Dye-decolorizing peroxidases (DyPs) are heme proteins with distinct structural properties and substrate specificities compared to classical peroxidases. Here, we demonstrate that DyP from the extremely radiation-resistant bacterium Deinococcus radiodurans is, like some other homologues, inactive at physiological pH. Structurally, DyP-type peroxidases also differ from the classical peroxidases. In contrast with the α-helix rich structures of the latter, DyPs are organized in two domains with a ferredoxin-like fold of four anti-parallel β-sheets surrounded by α-helices. A sequence analysis of DrDyP compared to four characterized and structurally determined members of the class V peroxidase family of DyPs, demonstrates that the proximal His heme ligand, and the four residues that are proposed to form the hydrogen peroxide binding pocket within this family of DyPs are conserved in DrDyP (H324, D189, R348, L373 and F375).

However, the so-called DyP fingerprint motif GXXDG has a substitution in the fifth position, containing a Methionine (M190) instead of a Glycine, as observed for the other DyPs. The proximity of this residue to the catalytic residue Asp189 made us suspect that it might affect the activity of the protein; we, thus, re-engineered a typical DyP distal site by generating the DrDyPM190G mutant for spectroscopic analysis. UV-vis and RR spectroscopies reveal that the resulting DrDyPM190G is also in a 6cLS spin state at pH 7.5, and thus the Methionine does not affect the activity of the protein. The E°′ of DrDyP and DrDyPM190G are found to be –81 ± 4 mV and −96 ± 7 mV, respectively, at pH 7.0, which we attribute to the 6cLS heme species, which is the major population present in the solution in both cases (cf. RR section). To gain more insight into the function of DyP from D. radiodurans, both DrDyP and DrDyPM190G were crystallized and structurally determined to 2.20 and 1.53 Å resolution, respectively. DrDyP possesses one and DrDyPM190G possesses two molecules in the asymmetric unit, respectively. Each molecule of the DrDyPM190G (residue 15–460) contains one heme molecule, one calcium (Ca), one Cl, one hydroxyl (OH), and 632 waters. The high-resolution structure of DrDyPM190G, obtained at pH 8.5, shows that one hydroxyl group and one water molecule are within hydrogen bonding distance to the heme and the catalytic Asparagine and Arginine. This strong ligand most likely prevents the binding of the H2O2 substrate, reinforcing questions about physiological substrates of this and other DyPs, and about the possible events that can trigger the removal of the hydroxyl group conferring catalytic activity to DrDyP. Here, we suggest that the presence of the hydroxyl group and the water molecule at the distal side of the heme iron can explain the hexacoordinated low-spin (6cLS) state of the heme of DrDyP, and thus the lack of activity of DrDyP at physiological pH.

>[2x]HNDKIDLDLDDIQATVLRERPEPYYGTHAMVRFDTAEGGRELLKRLLPHIASAEKWWDVKYAWTAAAISYEGLKKLGVPQDSLDSFPESFKVGMAGRAEHLFDVGENDPKHWEKPFGTGQVHLALTIFAENEENWQKALVIAEHELGATKGVTLLMREDFGAQPDSRNSLGYKDGISNPAIEGSGIKPFPGQGPAIKPGEFVLGYPGEAGVPLGMPKPEVLGKNGTFVALRKYHTNAGSFNRYLKENAEYTGGDAELLAAKLVGRWRSGAPLTLAPKEDDPELGHDPNRNNDFTYKNDPEGLEVPLGSHIRRMNPRDTKLELLTDVNIHRIIRRATAYGPAYDPKADSLAEDKVERGLYFIFISAKAMDTTEFLQKEWINKANFIGQGSERDPIVGLQDEDLTFTLPKEPVRQRLRGMDTFNVLRGGEYLFMPSLSALKWLSELK> SVLRTITNLQKKIRKELKQR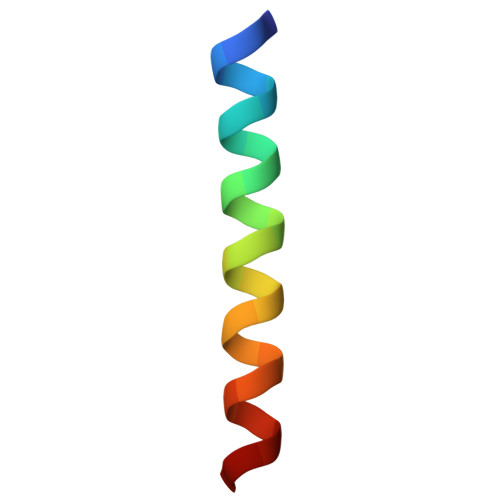QLKQE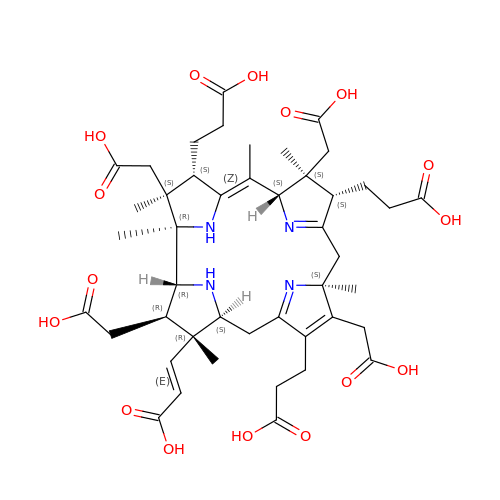3-[(1R,2S,3S,7S,11S,16S,17R,18R,19R)-2,7,12,18-tetrakis(2-hydroxy-2-oxoethyl)-3,13-bis(3-hydroxy-3-oxopropyl)-1,2,5,7,11,17-hexamethyl-17-(3-oxidanyl-3-oxidanylidene-prop-1-enyl)-3,6,8,10,15,16,18,19,21,24-decahydrocorrin-8-yl]propanoic acid | C45 H60 N4 O16 | DZSBRGWVIYKASI-BKOIVCMISA-N>GGMGQTLLDALNVRVVGSGERVLVLAHGFGTDQSAWNRILPFFLRDYRVVLYDLVCAGSVNPDFFDFRRYTTLDPYVDDLLHILDALGIDQCAYVGHSVSAMIGILASIRRPELFSKLILIGASPRFLNDEDYHGGFEQGEIEKVFSAMEANYEAWVNGFAPLAVGADVPAAVREFSRTLFNMRPDITLFVSRTVFNSDMRGVL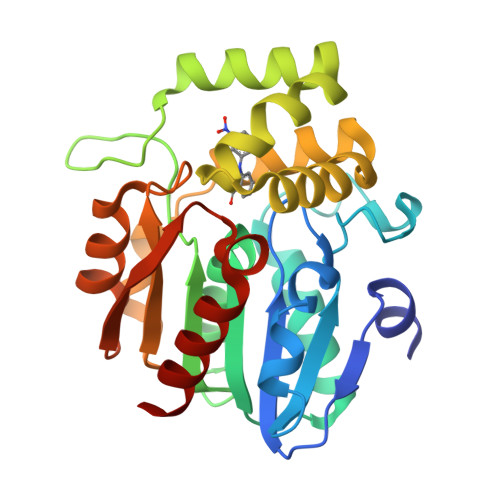GLVKVPCHIFQTARDHSVPASVATYLKNHLGGKNTVHWLNIEGHLPHLSAPTLLAQELRRALSHR[2x]>[2x]MAEEHHHHHHHHLEVLFQGPLRPRLCTMKKGPSGYGFNLHSDKSKPGQFIRSVDPDSPAEASGLRAQDRIVE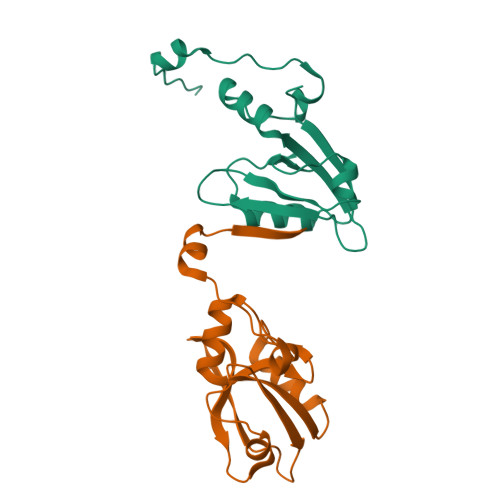VNGVCMEGKQHGDVVSAIRAGGDETKLLVVDRETDEFFKKCRVIPSQEHLNGPLPVPFTNGEIQKENSDTRL>MGAAAKLAFAVFLISCSSGAILGRSETQECLFFNANWEKDRTNQTGVEPCYGDKDKRRHCFATWKNISGSIEIVKQGCWLDDINCYDRTDCVEKKDSPEVYFCCCEGNMCNEKFSYFPEME[4x];>[4x]GLECDGKVNICCKKQFF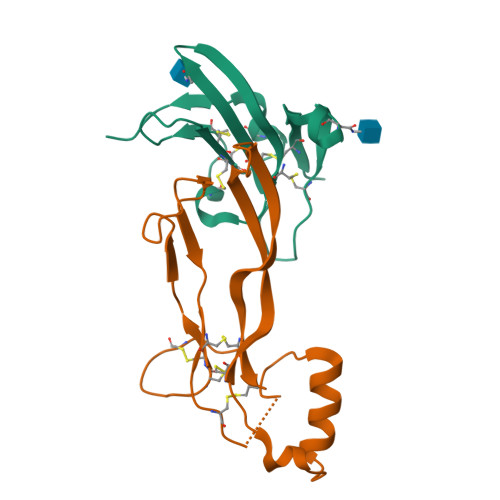VSFKDIGWNDWIIAPSGYHANYCEGECPSHIAGTSGSSLSFHSTVINHYRMRGHSPFANLKSCCVPTKLRPMSMLYYDDGQNIIKKDIQNMIVEECGCS Superoxide dismutases (SODs) are important enzymes in defence against oxidative stress. However, in 1996 a Plasmodium falciparum iron-dependent SOD (PfFeSOD) was identified in parasites isolated from infected blood cells. Malaria parasites are particularly prone to oxidative damage in the intra-erythrocytic stage of their lifecycle. The fact that it is an FeSOD and distinct from human tetrameric Mn and Cu/ZnSODs raises the possibility of its exploitation as an anti-malarial drug target and indeed inhibitors of PfFeSOD have been identified.

The crystal structure of PfFeSOD has been solved and refined against data extending to 2.5 Å spacing. The refined model consists of two polypeptide chains, A and B, which are related by a non-crystallographic two-fold axis of symmetry, together with two iron ions and 140 solvent water molecules. The overall structure is similar to those of previously solved iron superoxide dismutases, consisting of an amino terminal α-helical domain linked to a carboxy terminal α/β domain. Since the calculated molecular weight of the monomer is 23,799 Da, this indicates that PfFeSOD is a dimer, consistent with previously characterised FeSODs, which are either dimers or tetramers. The metal ion in both subunits of the enzyme is five-coordinate. The coordination geometry is trigonal bipyramidal, with His73, His161 and Asp157 providing the equatorial ligands and with His26 and the hydroxide or water oxygen atom forming the axial ligands. Trp122 forms a hydrogen bond to Gln69, which in turn forms a hydrogen bond with the hydroxyl group of Tyr34. Tyr34 is also hydrogen bonded via a water molecule to His30, which is bonded to Tyr134 from the other subunit. This classical hydrogen-bonding network in superoxide dismutases may allow communication between the two metal sites. There is an interesting pair of adjacent charge-charge interactions between the carboxylates of the Asp140 residues and the side chain imidazoles of His139.

>[2x]MVITLPKLKYALNALSPHISEETLNFHYNKHHAGYVNKLNTLIKDTPFAEKSLLDIVKESSGAIFNNAAQIWNHTFYWDSMGPDCGGEPHGEIKEKIQEDFGSFNNFKEQFSNILCGHFGSGWGWLALNNNNKLVILQTHDAGNPIKDNTGIPILTCDIWEHAYYIDYRNDRASYVKAWWNLVNWNFANENLKKAMQKLEHHHHHH PYRIMIDINE | C4 H4 N2 | 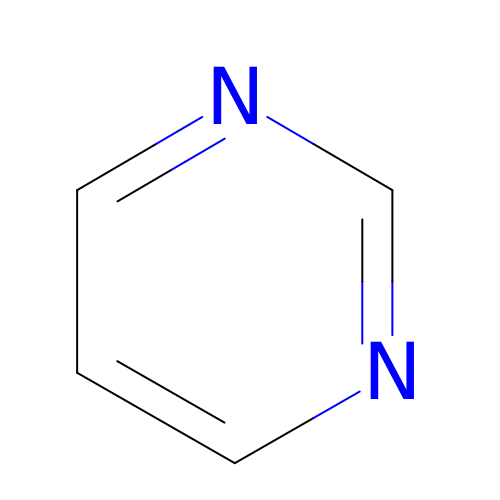CZPWVGJYEJSRLH-UHFFFAOYSA-N> GSQDPTIFEERHLKYISQLGKGNFGSVELCRYDPLGDNTGALVAVKQLQHSGPDQQRDFQREIQILKALHSDFIVKYRGVSYGPGRQSLRLVMEYLPSGCLRDFLQRHRARLDASRLLLYSSQICKGMEYLGSRRCVHRDLAARNILVESEAHVKIADFGLAKLLPLDKDYYVVREPGQSPIFWYAPESLSDNIFSRQSDVWSFGVVLYELFTYCDKSCSPSAEFLRMM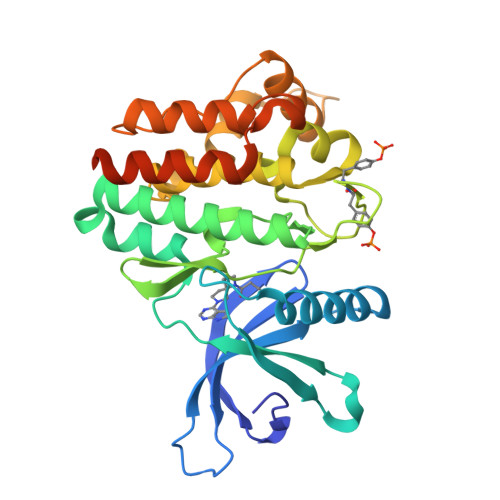GCERDVPALCRLLELLEEGQRLPAPPACPAEVHELMKLCWAPSPQDRPSFSALGPQLDMLWSGSRGCETHAFTAHPEGKHHSLSFS> GHMIHAISAVNRHLYEDVLEQHFRLRHDIFVEERHWETLRRPDGREVDSYDDEDTVYLLALEGRRVVGGHRLYPTTKPSMMSEVFPHLAAVRGCPSDPLIWEWSRYFVVRDRRDGALNLQLMAAVQEFCLDQGIAQVSAIMETWW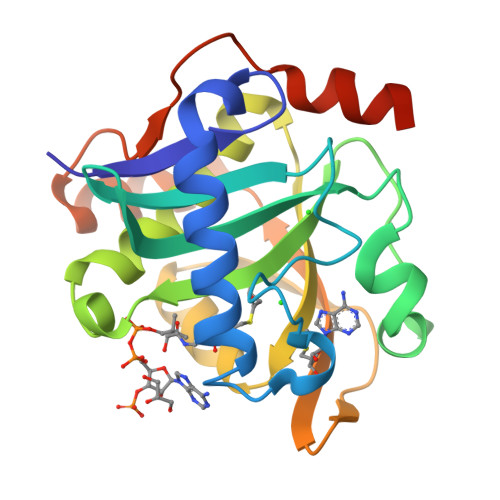LPRFHEAGFVVTPLGLPALVENAWTMAATVDIRRQTLDVLHDRIGMPSIVQQDGPRLDAVARANLCGLAAAQRKSA> GQVANTRIYAAEKLAKVKEKADSPLYAPAVKTLLRDADKALKMTPPSVMDKTMTADSGDKHDYMSMGPYWWPDPSKPDGLPYIRKDGQRNPELDKLDRNKLGDMSKAVTTLGLAYYFSGDEKYAQKAVDFLNVWFLDAKTKMNPHLTYGQTIPGKNKGMGRGAGMIDIYSFTEMIDAMTLMENSKAFTPKVKKGMKEWFTQLVEWMQTSPVAAEEQRAKNNHGLAYDVQLTAYALYTGNQDLAMKTIQEFPEKRLFAQIEPDGKQPLELA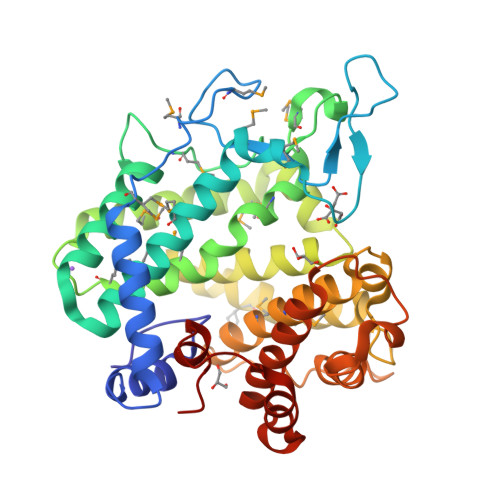RTTALGYTIFNLGHMLDMCSIASTLGQDIYNATSQDGRSITAALKFLIPYIGKPQSEWPYQQIKEWDKKQEEACWILRRASFFDPKAGYEAIGAQFRETPANKRIHLIYSLE2,2,7-TRIMETHYL-GUANOSINE-5'-TRIPHOSPHATE-5'-GUANOSINE 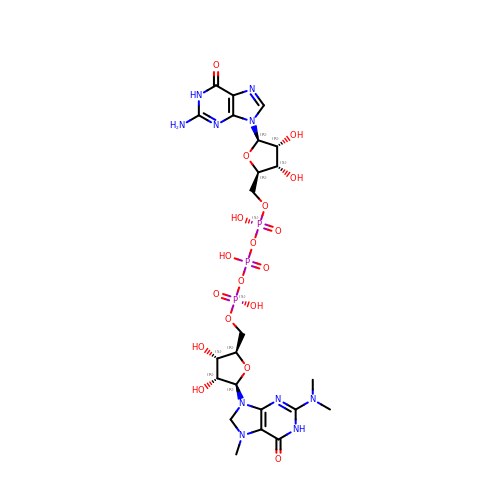| C23 H35 N10 O18 P3 | QBEUSSFUVVPDGT-NAGRZYTCSA-N>[7x]MSNETIVIDIKGAVQHPGVYEMRTGDRVSQAIEKAGGTSEQADEAQVNLAEILQDGTVVYIPKKGEETAVQQGGGGSVQSDGGKGALVNIN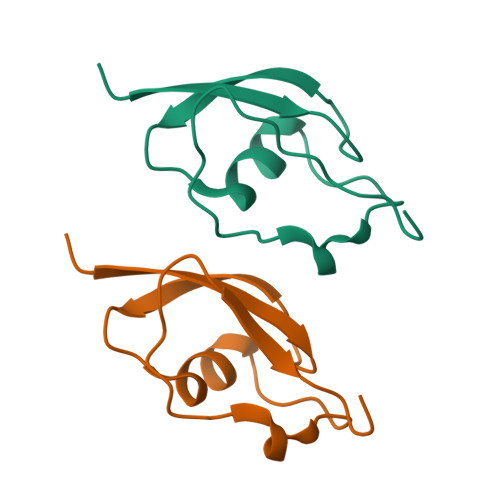TATLEELQGISGVGPSKAEAIIAYREENGRFQTIEDITKVSGIGEKSFEKIKSSITVKLEHHHHHH>[10x]DYKDDDDKLEVLFQGPGSLPVIAELPPKVSVFVPPRDGFFGNPRKSKLICQATGFSPRQIQVSWLREGKQVGSGVTTDQVQAEAKESGPTTYKVTSTLTIKESDWLGQSMFTCRVDHRGLTFQQNASSMCVPDQDTAIRVFAIPPSFASIFLTKSTKLTCLVTDLTTYDSVTISWTRQNGEAVKTHTNISESHPNATFSAVGEASICEDDWNSGERFTCTVTHTDLPSPLKQTISRPKGVALHRPDVYLLPPAREQLNLRESATITCLVTGFSPADVFVQWMQRGQPLSPEKYVTSAPMPEPQAPGRYFAHSILTVSEEEWNTGETYTCVVAHEALPNRVTERTVDKSTGKPTLYNVSLVMSDTAGTCY;> KSPIFGPEEVNSVEGNSVSITCYYPPTSVNRHTRKYWCRQGARGGCITLISSEGYVSSKYAGRANLTNFPENGTFVVNIAQLSQDDSGRYKCGLGINSRGLSFDVSLEVSQGPGLLNDTKVYTVDLGRTVTINCPFKTENAQKRKS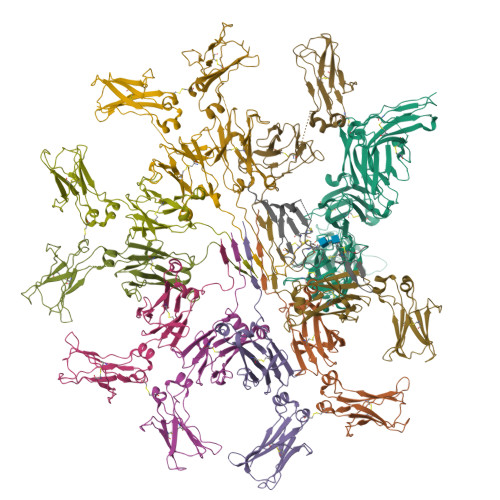LYKQIGLYPVLVIDSSGYVNPNYTGRIRLDIQGTGQLLFSVVINQLRLSDAGQYLCQAGDDSNSNKKNADLQVLKPEPELVYEDLRGSVTFHCALGPEVANVAKFLCRQSSGENCDVVVNTLGKRAPAFEGRILLNPQDKDGSFSVVITGLRKEDAGRYLCGAHSDGQLQEGSPIQAWQLFVNEESTIPRSPTVVKGVAGGSVAVLCPYNRKESKSIKYWCLWEGAQNGRCPLLVDSEGWVKAQYEGRLSLLEEPGNGTFTVILNQLTSRDAGFYWCLTNGDTLWRTTVEIKIIEGEPNLKVPGNVTAVLGETLKVPCHFPCKFSSYEKYWCKWNNTGCQALPSQDEGPSKAFVNCDENSRLVSLTLNLVTRADEGWYWCGVKQGHFYGETAAVYVAVEERKAAGSRDVSLAKADAAPDEKVLDSGFREIENKAIQDPRHHHHHH;> QEDERIVLVDNKCKCARITSRIIRSSEDPNEDIVERNIRIIVPLNNRENISDPTSPLRTRFVYHLSDLCKKCDPTEVELDNQIVTATQSNICDEDSATETCYTYDRNKCYTAVVPLVYGGETKMVETALTPDACYPD> MVSFKAGINLGGWISQ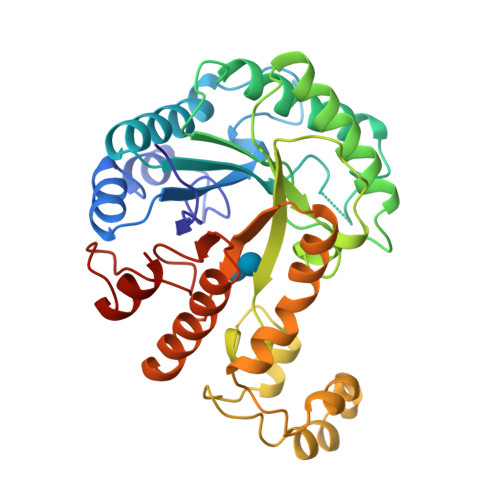YQVFSKEHFDTFITEKDIETIAEAGFDHVRLPFDYPIIESDDNVGEYKEDGLSYIDRCLEWCKKYNLGLVLDMHHAPGYRFQDFKTSTLFEDPNQQKRFVDIWRFLAKRYINEREHIAFELLNQVVEPDSTRWNKLMLECIKAIREIDSTMWLYIGGNNYNSPDELKNLADIDDDYIVYNFHFYNPFFFTHQKAHWSESAMAYNRTVKYPGQYEGIEEFVKNNPKYSFMMELNNLKLNKELLRKDLKPAIEFREKKKCKLYCGEFGVIAIADLESRIKWHEDYISLLEEYDIGGAVWNYKKMDFEIYNEDRKPVSQELVNILARRKT>[2x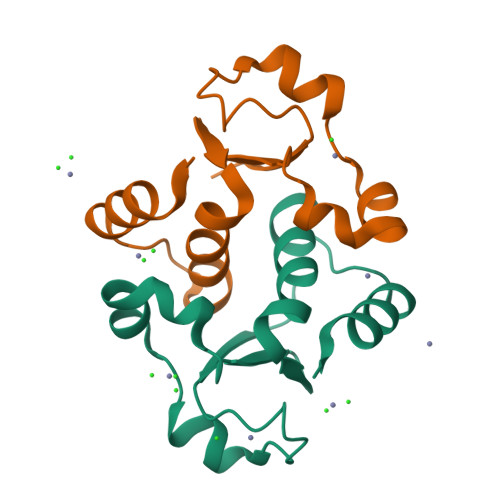]SLRDLPSIAISLCGGLSDHREITKDAFLEQAVSYQQFADNPAIIDDPNLVVKVGNKYYNWTTAAPLLLAMQAFQKPLPKATVESIMRDKMP>MIAQ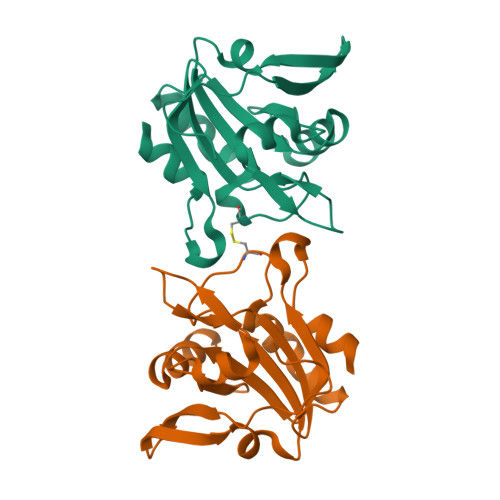GQTLPNATLSQLTKEGMVHHPVLELFAGKKVVLFAVPGAFTPTCSEAHLPGYIVLADQLKAKGVDLIASVSVNDAFVMKAWGEAQNAEEILMLADGDASFTKALGLEMDTAGFGGLRSQRYAMIIDNGVVTTLNVEAPKSFEVSNAETILAALEHHHHHH[2x]> PKDAQVIMSILKELNVQEYEPRVVNQLLEFTFRYVTS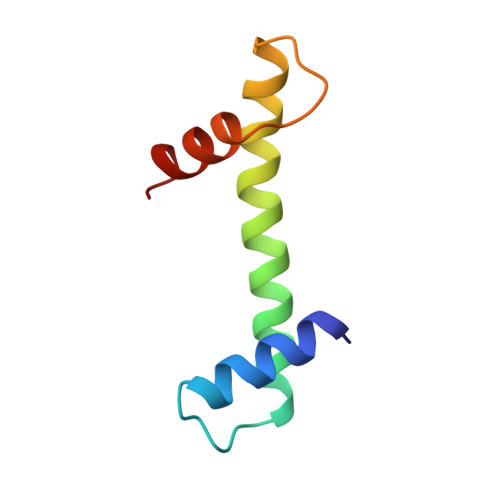ILDDAKVYANHARKKTIDLDDVRLATEVTLD>GSHMRHRTLSSSPALWASIPCPRSELRLDLVLASGQSFRWKEQSPAHWSGVLADQVWTLTQTEDQLYCTVYRGDDSQVSRPTLEELETLHKYFQLDVSLAQLYSHWASVDSHFQRVAQKFQGVRLLRQDPTECLFSFICSSNNNIARITGMVERLCQAFGPRLIQLDDVTYH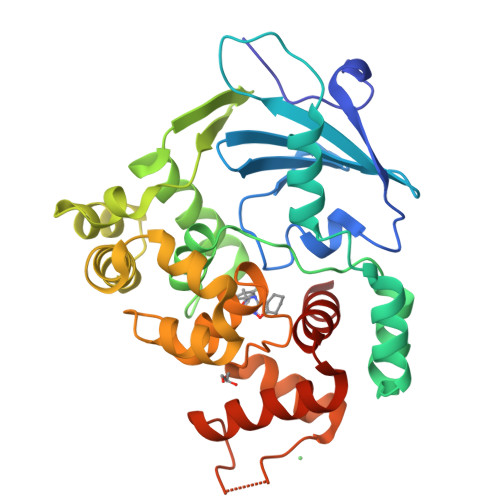GFPNLHALAGPEAETHLRKLGLGYRARYVRASAKAILEEQGGPAWLQQLRVAPYEEAHKALCTLPGVGAKVADCICLMALDKPQAVPVDVHVWQIAHRDYGWHPKTSQAKGPSPLANKELGNFFRNLWGPYAGWAQAVLFSADLRQ[3x]1-methyl-1,2-dihydro-3H-indol-3-one | C9 H9 N O | 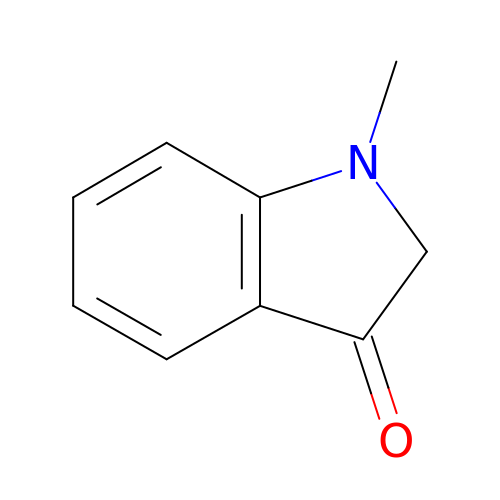DYPFVQQCYZKNMK-UHFFFAOYSA-N>[2x]GFLSGKRILVTGVASKLSIAYGIAQAMHREGAELAFTYQNDK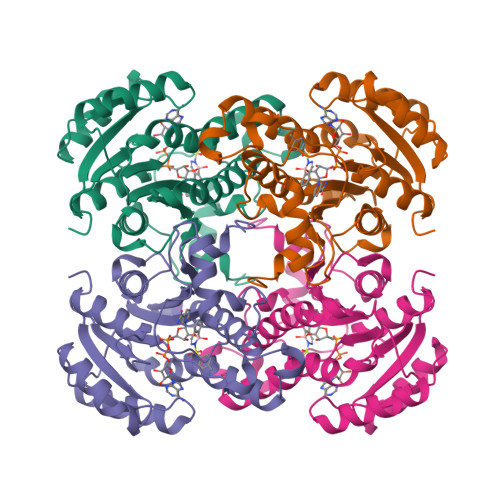LKGRVEEFAAQLGSDIVLQCDVAEDASIDTMFAELGKVWPKFDGFVHSIGFAPGDQLDGDYVNAVTREGFKIAHDISSYSFVAMAKACRSMLNPGSALLTLSYLGAERAIPNYNVMGLAKASLEANVRYMANAMGPEGVRVNAISAGPIRTLAASGIKDFRKMLAHCEAVTPIRRTVTIEDVGNSAAFLCSDLSAGISGEVVHVDGGFSIAAMNELELK> MELHQIRGCHKNDIELKKYNIGVAISLGNKWFSIDNIEKLVKWSLLHTKEYVIIFIADSIHGINLSVRNKLSDSHAEEVAIRYGRNLFIKIKERVSLSFSQDEQAKIIYATWSDIADSKYKEKVKYLYNLYDKNINFKNYIENFVKEWVSKEKRTFNNNEINKFGRYILEELPELMVQVKARGVLFEAYVYPYKTRITEFVGLL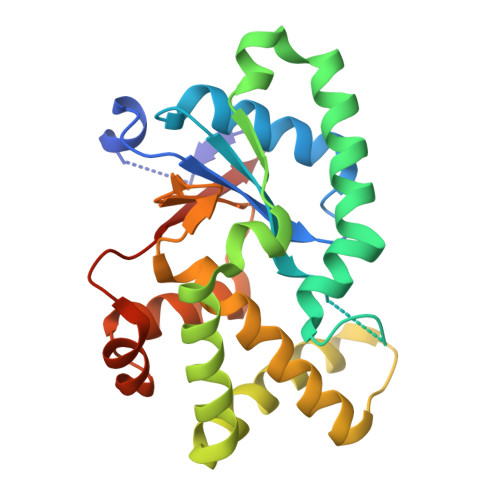QKGEIFPEIKTNILDNHPKIFLEVREHHHHHH> QAQITGRPEWIWLALGTALMGLGTLYFLVKGMGVSDPDAKKFYAITTLVPAIAFTMYLSMLLGYGLTMVPFGGEQNPIYWARYADWLFTTPLLLLDLALLVDADQGTILALVGADGIMIGTGLVGALTKVYSYRFVWWAISTAAMLYILYVL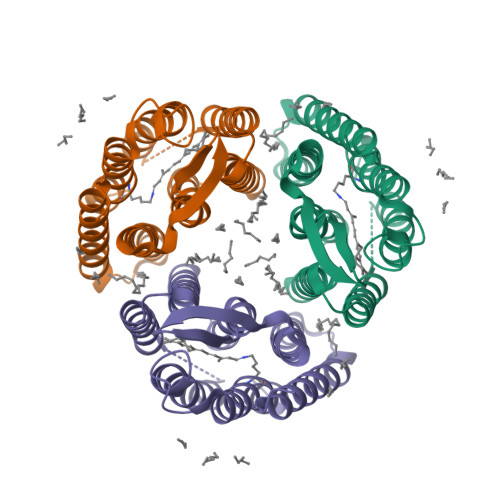FFGFTSKAESMRPEVASTFKVLRNVTVVLWSAYPVVWLIGSEGAGIVPLNIETLLFMVLDVSAKVGFGLILLRSRAIFGEAEAPEPSAGDGAAATS> MRGSHHHHHHTDQFTMEQNPQSQLKLLVTRGKEQGYLTYAEVNDHLPEDIVDSDQIEDIIQMINDMGIQVMEEAPDADDLMLAENTADEDAAEAAAQVLSSVESEIGRTTDPVRMYMREMGTVELLTREGEIDIAK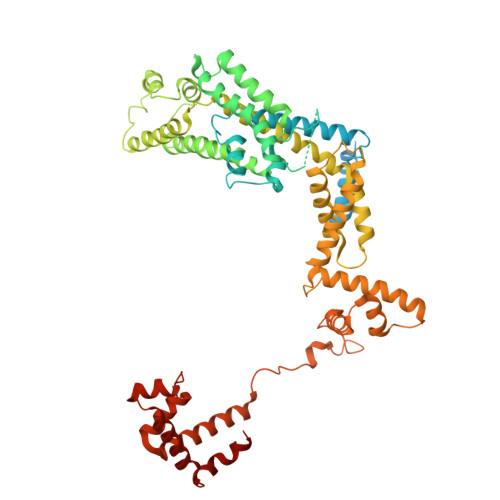RIEDGINQVQCSVAEYPEAITYLLEQYDRVEAEEARLSDLITGFVDPNAEEDLAPTATHVGSELSQEDLDDDEDEDEEDGDDDSADDDNSIDPELAREKFAELRAQYVVTRDTIKAKGRSHATAQEEILKLSEVFKQFRLVPKQFDYLVNSMRVMMDRVRTQERLIMKLCVEQCKMPKKNFITLFTGNETSDTWFNAAIAMNKPWSEKLHDVSEEVHRALQKLQQIEEETGLTIEQVKDINRRMSIGEAKARRAKKEMVEANLRLVISIAKKYTNRGLQFLDLIQEGNIGLMKAVDKFEYRRGYKFSTYATWWIRQAITRSIADQARTIRIPVHMIETINKLNRISRQMLQEMGREPTPEELAERMLMPEDKIRKVLKIAKEPISMETPIGDDEDSHLGDFIEDTTLELPLDSATTESLRAATHDVLAGLTAREAKVLRMRFGIDMNTDYTLEEVGKQFDVTRERIRQIEAKALRKLRHPSRSEVLRSFLDD> SRNICYDAFVS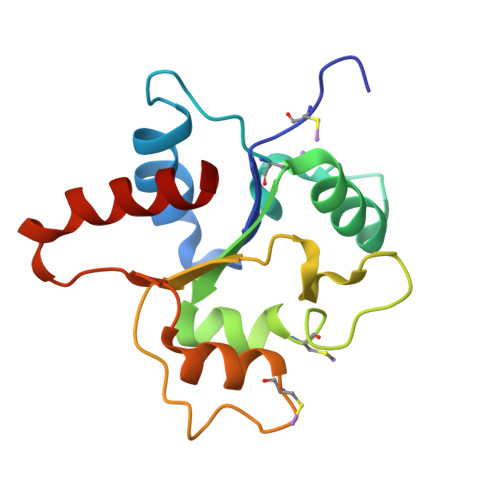YSERDAYWVENLMVQELENFNPPFKLCLHKRDFIHGKWIIDNIIDSIEKSHKTVFVLSENFVKSEWCKYELDFSHFRLFDENNDAAILILLEPIEKKAIPQRFCKLRKIMNTKTYLEWPMDEAQREGFWVNLRAAIKS> MENFPIISLDKVNGVERAATMEMIKDAC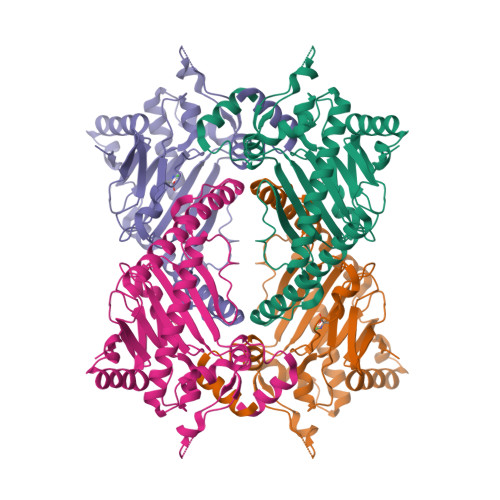ENWGFFELVNHGIPREVMDTVEKMTKGHYKKCMEQRFKELVASKALEGVQAEVTDMDWESTFFLKHLPISNISEVPDLDEEYREVMRDFAKRLEKLAEELLDLLCENLGLEKGYLKNAFYGSKGPNFGTKVSNYPPCPKPDLIKGLRAHTDAGGIILLFQDDKVSGLQLLKDGQWIDVPPMRHSIVVNLGDQLEVITNGKYKSVMHRVIAQKDGARMSLASFYNPGSDAVIYPAPALVEKEAEENKQVYPKFVFDDYMKLYAGLKFQAKEPRFEAMKAMETDVKMDPIATV(2E,4E,6Z,8E)-3,7-dimethyl-8-[2-(3-methylbutyl)-3-propylcyclohex-2-en-1-ylidene]octa-2,4,6-trienoic 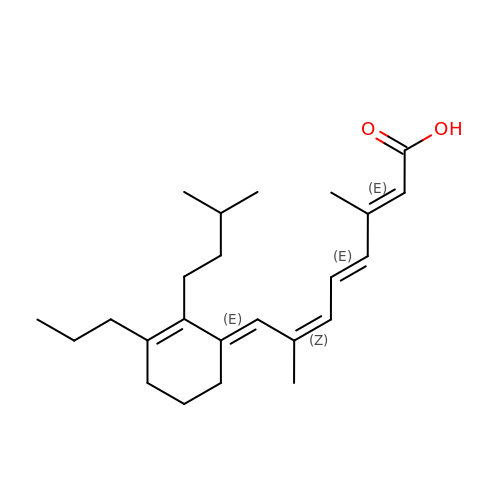acid | C24 H36 O2 | AFPIKPIXJYHWHZ-JALBNXGMSA-N>[4x]MKKIEAIIKPFKLDEVKDALVEIGIGGMTVTEVKGFGQQKGHTEIYRGT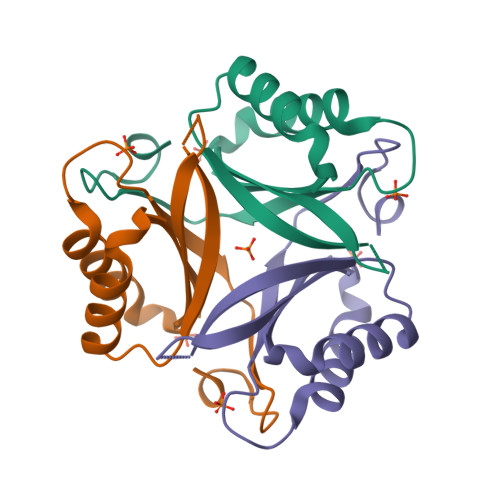EYVIDFLPKVKIEVVVRDEDVEKVVETIVKTAQTGRVGDGKIFIIPVEDVIRIRTGERGEQAI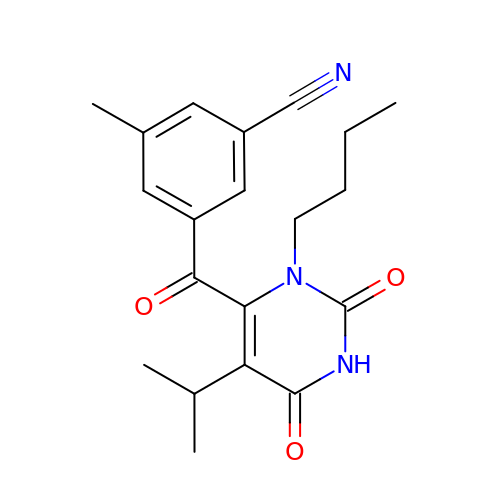3-{[3-butyl-5-(1-methylethyl)-2,6-dioxo-1,2,3,6-tetrahydropyrimidin-4-yl]carbonyl}-5-methylbenzonitrile | C20 H23 N3 O3 | PPJRWFFVCKGABJ-UHFFFAOYSA-N5-phenyluridine 5'-(trihydrogen diphosphate) | C15 H18 N2 O12 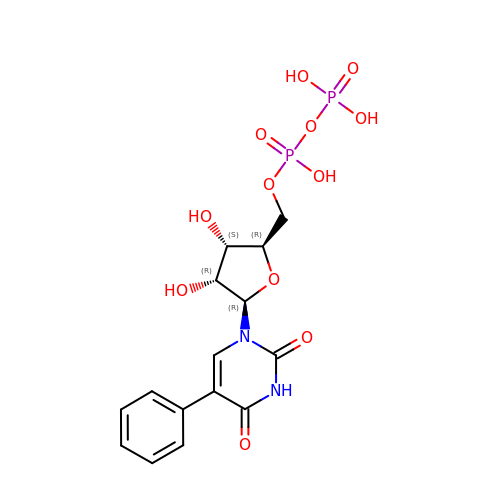P2 | YEGUYIFHFHBENO-HKUMRIAESA-N> GSRLSVAPEMDIMDYCKKEWRGNTQKATCMK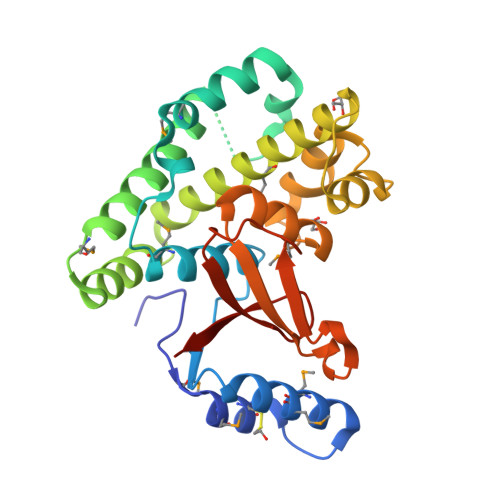MGYEEVSQKFTSIRRVRGDNYCALRATLFQAMSQAVGLPPWLQDPELMLLPEKLISKYNWIKQWKLGLKFDGKNEDLVDKIKESLTLLRKKWAGLAEMRTAEARQIACDELFTNEAEEYSLYEAVKFLMLNRAIELYNDKEKGKEVPFFSVLLFARDTSNDPGQLLRNHLNQVGHTGGLEQVEMFLLAYAVRHTIQVYRLSKYNTEEFITVYPTDPPKDWPVVTLIAEDDRHYNIPVRVCEETSL>MASMTGGQQMGR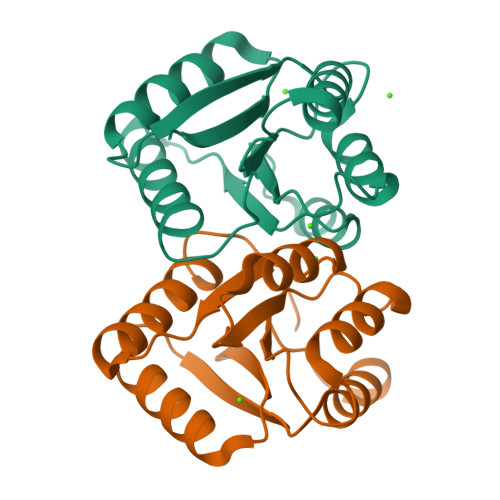GSMPERASVPLRLLLVEDNAADIFLMEMALEYSSVHTELLVARDGLEALELLEQAKTGGPFPDLILLDLNMPRVDGFELLQALRADPHLAHLPAIVLTTSNDPSDVKRAYALQANSYLTKPSTLEDFLQLIERLTAYWFGTAAIPQTYQPQLEHHHHHH[4x]>[12x]ADPAPTSSSTKKTQLQLEHLLLDLQMILNGINNYKNPKLTRMLTFKFYMPKKATELKHLQCLEEELKPLEEVLNLAHSKNFHFDPR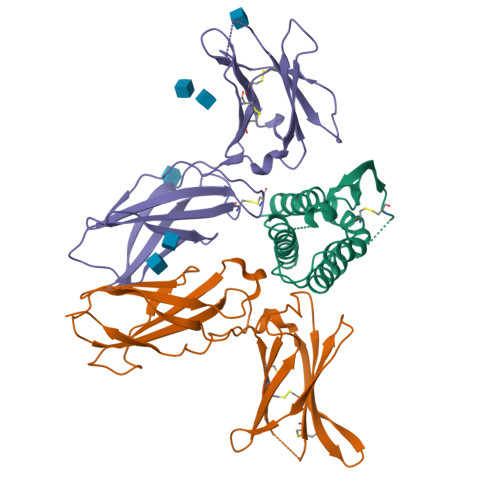DVVSNINVFVLELKGSETTFMCEYADETATIVEFLNRWITFCQSIISTLT;>[12x]ADPAVQGTSQFTCFYNSRAQISCVWSQDGALQDTSCQVHAWPDRRRWQQTCELLPVSQASWACNLILGAPDSQKLTTVDIVTLRVLCREGVRWRVMAIQDFKPFENLRLMAPISLQVVHVETHRCNISWEISQASHYFERHLEFEARTLSPGHTWEEAPLLTLKQKQEWICLETLTPDTQYEFQVRVKPLQGEFTTWSPWSQPLAFRTKPAALGKDT;>[12x]ADPPLPEVQCFVFNVEYMNCTWQSSSEPQPTNLTLHYWYKNSDNDKVQKCSHYLFSEEITSGCQLQKKEIHLYQTFVVQLQDPREPRRQATQMLKLQNLVIPWAPENLTLHKLSESQLELNWNNRFLNHCLEHLVQYRTDWDHSWTEQSVDYRHKFSLPSVDGQKRYTFRVRSRFNPLCGSAQHWSEWSHPIHWGSNTSKEN>EVKLILYHWTHSFSSQKVRLVIAEKALKCEEHDVSLPLSEHNEPWFMRLNSTGEVPVLIHGENIICEATQIIDYLEQTFLDERTPRLMPDKESMYYPRVQHYRELLDSLPMDAYTHGCILHPELTVDSMIPAYATTRIRSQIGNTESELKKLAEENPDLQEAYIAKQKRLKSKLLDHDNVKYLKKILDELEKVLDQVETELQRRNEETPEEGQQPWLCGESFTLVDVSLAVTLHR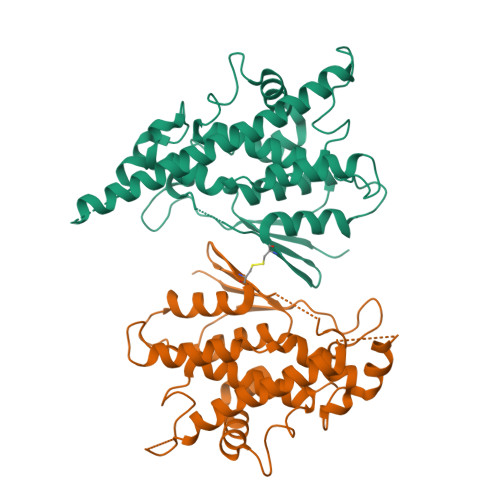LKFLGFARRNWGNGKRPNLETYYERVLKRKTFNKVLGHVNNILIS[2x]>MVLKLYAVSDGPPSLSVRQALVALEVPFELINVDFGAGEHMTSDYALMNPQKEIPVLDDEGFYLSESNAILQYICDKYRPGSPLYPQDPKSRAIVNHRLCFNLSSYYANISAYTMAPIFFDYERTPLGLKKVHISLDVLETYLTRTNTSYAAANHLTIADFPLINSTMTLEAIDFDFSKYTKIHKWYNDFKVKYPDLWKISESAMKEIQHFAANPPDLTHLNHPIHPIRKIKN[2x]

Glutathione (GSH) S-transferases (GSTs, EC 2.5.1.18) are cytosolic enzymes that are present in both prokaryotes and eukaryotes. GSH conjugation is essential for the detoxification of xenobiotics. Previously, we identified a novel GST obtained from B. mori (bmGSTu2). We also found that bmGSTu2 was capable of metabolising diazinon.

The crystal structure of bmGSTu2 was determined at 1.68 Å resolution and solved by the single-wavelength anomalous diffraction (SAD) method using the Hg-derivative. The purified protein was crystallised in a space group of P41 with unit cell dimensions a = b = 86.26 Å and c = 58.77 Å. Structural elements, characterised by the STRIDE program for protein secondary structure assignment, showed that bmGSTu2 contains 8 α-helices and 4 β-strands. Two discrete domains, N-terminal (residues 1–78) and C-terminal (residues 89–233), were connected by a linker region (residues 79–88). Similar to other GSTs, the bmGSTu2 structure adopted the canonical GST fold. Superposition of the structure of bmGSTu2 onto that of nlGSTD demonstrated that the α-helices and β-strands of bmGSTu2 were conserved across the structures. For GSH activation, an electron-sharing network was proposed for a delta-class GST in Anopheles dirus (adGSTD3–3), and the network includes Glu64, Ser65, Arg66, Asp100, Thr158, and Thr16221,22. The corresponding residues in bmGSTu2 are Glu66, Ser67, Asn68, Asn102, Pro162, and Ser166. In the bmGSTu2 structural model, the electron densities from the following regions were poor for modelling: Ala116 to Glu123, after Phe211 of the A chain, and from Pro117 to Tyr122. Our mutagenesis experiments indicate that the residues Pro13, Tyr107, Ile118, Phe119, and Phe211 in bmGSTu2 play important roles in its enzymatic functions. The decreased LD50 value observed for the mutant after diazinon exposure indicates that bmGSTu2 is involved in diazinon tolerance in vivo.DAMINOZIDE | C6 H12 N2 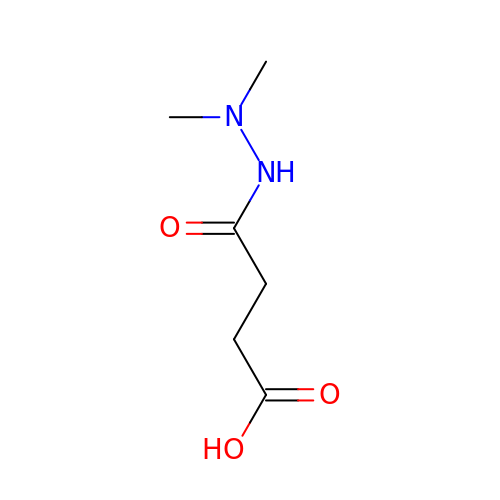O3 | NOQGZXFMHARMLW-UHFFFAOYSA-N> QANLMRLKSDLFNRSPMYPGPTKDDPLTVTLGFTLQDIVKVDSSTNEVDLVYYEQQRWKLNSLMWDPNEYGNITDFRTSAADIWTPDITAYSSTRPVQVLSPQIAVVTHDG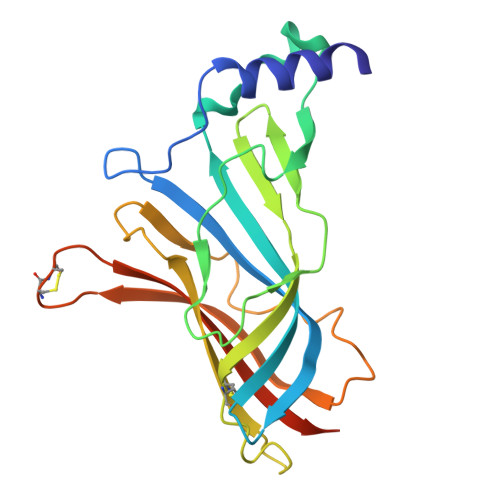SVMFIPAQRLSFMCDPTGVDSEEGVTCAVKFGSWVYSGFEIDLKTDTDQVDLSSYYASSKYEILSATQTRQVQHYSCCPEPYIDVNLVVKFRERRAGNGFFRNLFD> AISIKTPEDIEKMRVAGRLAAEVLEMIEPYVKPGVSTGELDRICNDYIVNEQHAVSACLGYHGYPKSVCISINEVVCHGIPDDAKLLKDGDIVNIDVTVIKDGFHGDTSKMFIVGKPTIMGERLCRITQESLYLALRMVKPGINLREIGAAIQKFVEAEGFSVVREYCGHGIGRGFHEEPQVLHYDSRETNVVLKPGMTFTIEPM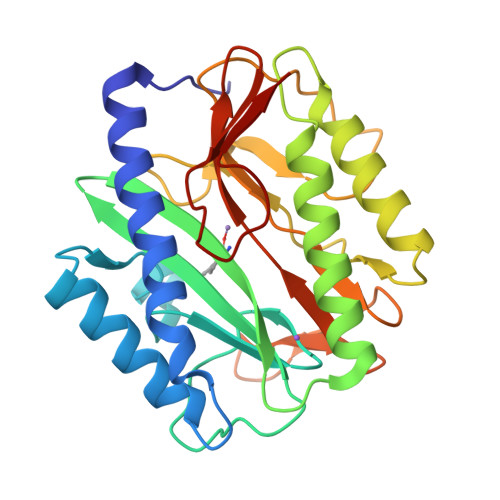VNAGKKEIRTMKDGWTVKTKDRSLSAQYEHTIVVTDNGCEILTLRKDDTIPAIISH> MSVVLTTIMNADQQLRYPSVGELEQIKNFMEDSALRLKVAKTLSDANDRV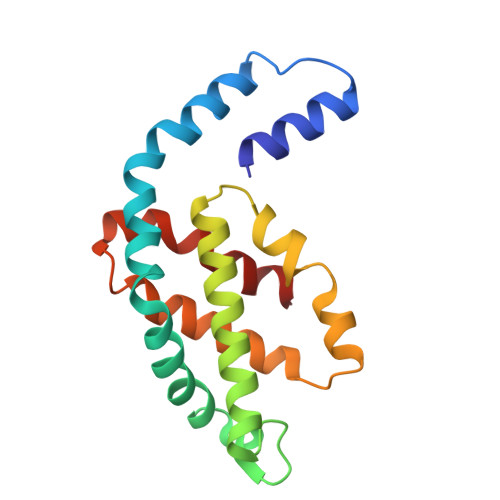VKQASAGLFQRRPDLNNPGGNAYGEKRLGSCIRDLGWYYRLITYSIVAGNNEPVERIGLTGIFEMYRVLEVPIPAMIESMRLLKKEALELLSPAEAEIAAPYFDYVIGAMQ The APTX RNA‐DNA deadenylase protects genome integrity and corrects abortive DNA ligation arising during ribonucleotide excision repair and base excision DNA repair, and APTX human mutations cause the neurodegenerative disorder ataxia with oculomotor ataxia 1 (AOA1). The aprataxin (APTX) RNA/DNA polynucleotide deadenylase directly reverses 5′‐AMP damage (Ahel et al, 2006; Harris et al, 2009; Reynolds et al, 2009; Tumbale et al, 2011, 2014) and associates with DNA repair scaffolds XRCC1 (Cherry et al, 2015) and XRCC4. Environmental and metabolic sources of DNA damage prompt “abortive ligation”, the failure of ligase to complete step 3, and generation of 5′‐adenylated (5′‐AMP) DNA strand breaks (Ahel et al, 2006; Andres et al, 2015; Schellenberg et al, 2015). AOA1 mutations map to the APTX catalytic domain (Barbot et al, 2001; Moreira et al, 2001; Shimazaki et al, 2002; Le Ber et al, 2003; Tranchant et al, 2003; Criscuolo et al, 2004, 2005; Ito et al, 2005; Mosesso et al, 2005; Baba et al, 2007; Yokoseki et al, 2011) and cause variable age of disease onset.

L248M: The dominant L248M APTX mutant was identified in AOA1 patients with severe clinical phenotype presenting early disease onset and a progressive ataxic syndrome with cerebellar atrophy, mental retardation, and epilepsy (Castellotti et al, 2011). This substitution is conservative and slightly stabilizing in the presence of AMP, yet unexpectedly has a ~7‐fold impact on APTX deadenylation at 37°C. Intriguingly, the crystal structure of L248M shows limited overall conformational perturbation of the DNA bound protein, with structural changes limited to minor shifts in neighboring His228. However, Leu248 maps to strand β4, is found in the protein hydrophobic core, and flanks regions of the protein undergoing conformational changes between the catalytic domain closed and opened states. These conformational changes extend from α1 to residues surrounding the active site and Leu248 also participates in this network. Thus, we hypothesized that L248M might impact solution conformational states of the protein. Consistent with this hypothesis, and in stark contrast to the DNA bound X‐ray structure of the L248M protein, apo L248M displayed significant global conformational perturbations in 1H‐15N HSQC spectra of unliganded protein compared to WT. Given the distance from the catalytic center (> 10 Å), we assert that L248M substitution impacts active site assembly allosterically, possibly through a network of interactions within the protein core that are influenced by this substitution. NMR results show the L248M mutation impacts a network of surrounding secondary structure, rendering the domain “arthritic”, such that DNA binding‐induced conformational changes are impaired. The stabilizing effect of L248M and its allosteric impact on catalytic domain conformations suggest that this mutation influences active site assembly and disassembly.

>GSHMGHWSQGLKISMQDPKMQVYKDEQVVVIKDKYPKARYHWLVLPWTSISSLKAVAREHLELLKHMHTVGEKVIVDFAGSSKLRFRMGYHAIPSMSHVHLHVISQDFDSPCLKNKKHWNSFNTEYFLESQAVIEMVQEAGRVTVRDGMPELLKLPLRCHECQQLLPSIPQLKEHLRKHWTQ[2x]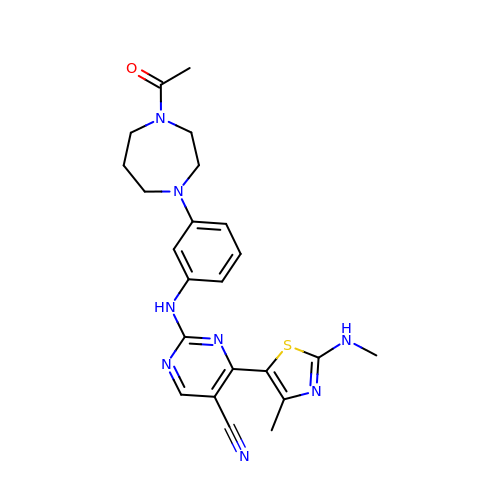2-[[3-(4-ethanoyl-1,4-diazepan-1-yl)phenyl]amino]-4-[4-methyl-2-(methylamino)-1,3-thiazol-5-yl]pyrimidine-5-carbonitrile | C23 H26 N8 O S | DZHBFQMOLIUZMP-UHFFFAOYSA-N> MSYSYIFKYIIIGDMGVGKSCLLHQFTEKKFMADCPHTIGVEFGTRIIEVSGQKIKLQIWDTAGLERFRAVTRSYYRGAAGALMVYDITRRSTYNHLSSWLTDARNLTNPNTVIILIGNKADLEAQRDVTYEEAKQFAEENGLLFLEASAKTGENVEDAFLEAAKKIYQNIQDGS;> MSDPAF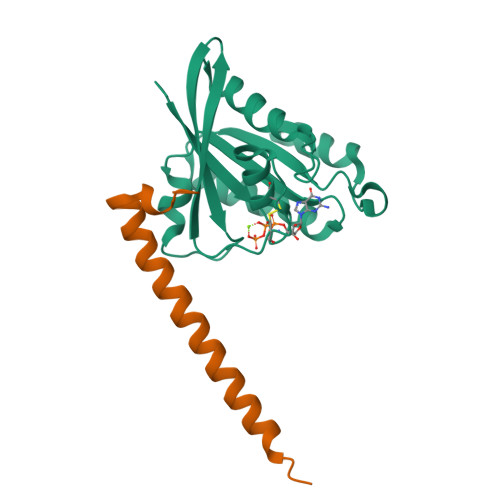AYAQLTHDELIQLVLKQKETISKKEFQVRELEDYIDNLLVRVMEETPNILRIPTQVGKKAGKM>[5x]RNAIEEKPLVVATKPSSEQYILGEILSLLLEKHHIPIKRAFGIGGGTMNIHPALIRGDFDLYVEYTGTAWVNTLKNPLTQKVDFETIKKRYEKEFNLLWVGLLGFNNTYSLAISKEDAQKYAIETFS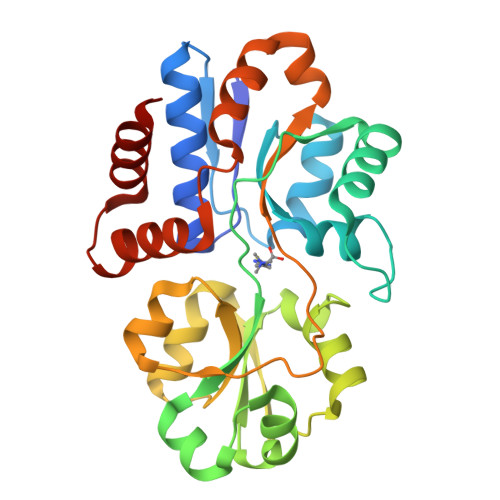DLAFHSPNFDFGAEFDFFEREDAFKGLMKAYRFHFRSLHEMDINLRYKSFESHKINALDVFTTDAQIKELDLKVLKDDKGFFPNYQAGIVIRKETIKKYPEALKILEKLDSKINDETMQDLNYQVEVLKKSPKIVAKDFLERLGL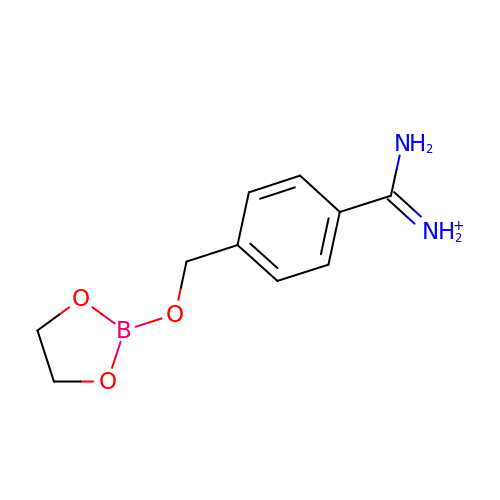[4-(1,3,2-DIOXABOROLAN-2-YLOXY)METHYL]BENZAMIDINE | C10 H14 B N2 O3 | XCLFQXCQQHVLJQ-UHFFFAOYSA-O> HHHHHMTKNYTEAQLKYYDANTGLCGIGIDQWFQYEPERNQFSTAFPLLFMLSELSLNSKEDTTAELYKNLNLRSEDEVVNVNQAVNTNLNTKNEVYQSTLILNAYTDIDSPFSETFIQNFAKVFNGTVKNIDYSNDAVATIRDSLQSDSGNDIEIALKDGDINKDTGIILTAYTNIYFPWGEASDSYRPYKQIDISFTALDGTQSNKQAWYSEGAGKYAEIENLGIKVFQFSLKPGLTVVLGTSLNDNNDLSGAFNKLRDPATLAYILTQTESKYLKLAVPIELTMRDSRDYIPEVKRAGLLTELFEKNFDGFDTVYDNKSGYISYMLSHTRLEFEQPTEEQAASVVAEPDFIFDKPYFFLVLDQFNTPAFIGLITN

Serpins play important roles in multiple processes, such as blood coagulation, fibrinolysis, tumor metastasis and immunity. Mature serpins usually contain 350–400 amino acids and share a conserved folding pattern that is mainly composed of eight or nine α-helices, three β-sheets, and a reactive center loop (RCL). The exposed RCL is located near the carboxyl-terminus, and it acts as bait for protease binding and cleavage. Three homologous serpins have been identified in the silk gland (a highly specialized organ that functions to synthesize and store silk proteins) of Bombyx mori: serpin16, serpin18, and serpin22.

To understand the physiological roles and inhibitory mechanism of these serpins, we determined the crystal structure of serpin18 at 1.65 Å. The overall fold of serpin18 resembles the canonical serpin conformation: an α/β fold consisting of one core β-sheets surrounded by nine α-helices (hA–hI) that are classified according to the conventional serpin nomenclature. Specifically, the segment with residues Glu352–Pro368 makes up the active RCL region, which is folded into a 1.5-turn helix (Glu355–Ser360) and two defined loops (Gln352–Thr354 and Gln361–Pro365, respectively). All residues of the RCL were well defined in the final electron density map, presumably because of the interaction between the RCL region and the underlying protein scaffold. The RCL in serpin18 is situated directly above of β-sheet C, and is closer to the core of the protein compared to those of the classical serpins. Further structural analysis showed that the RCL in serpin18 adopts a more stable conformation, presumably because of interactions between the RCL center region and β-sheet C. Furthermore, multiple-sequence alignment and structural analyses showed that the RCL in serpin18 is shorter by about 7 amino acids compared to that of the typical serpins. Notably, the length of the RCL up to the scissile bond in serpin18 is only 11 amino acids, whereas the length in other serpins is always 17 residues (P17–P1)23. Moreover, the papain-like mammalian cysteine protease, cathepsin L, was also inactivated by serpin18. These results demonstrated that serpin18 might act as a cysteine protease inhibitor, instead of as a serine protease inhibitor. In contrast, the inhibitory activities of the V362G and V362T mutants dramatically decreased, resulting in an extrapolated molar ratio of inhibitor-to-protease, which increased from ~1.3 for the wild-type to ~5–7 for the Val362 variants. This result confirmed the importance of Val362 at the reactive site of serpin18. Thus, we conclude that serpin18 plays a physiological role in regulating the activity of fibroinase and protecting silk proteins from degradation during B. mori development.> YEHTAVMPNKVGIPYK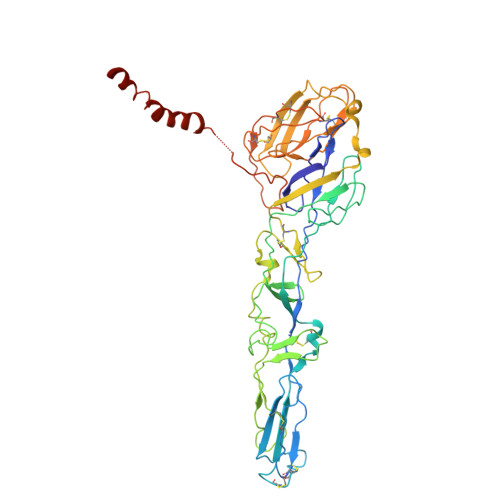ALVERPGYAPVHLQIQLVNTRIIPSTNLEYITCKYKTKVPSPVVKCCGATQCTSKPHPDYQCQVFTGVYPFMWGGAYCFCDTENTQMSEAYVERSEECSIDHAKAYKVHTGTVQAMVNITYGSVSWRSADVYVNGETPAKIGDAKLIIGPLSSAWSPFDNKVVVYGHEVYNYDFPEYGTGKAGSFGDLQSRTSTSNDLYANTNLKLQRPQAGIVHTPFTQAPSGFERWKRDKGAPLNDVAPFGCSIALEPLRAENCAVGSIPISIDIPDAAFTRISETPTVSDLECKITECTYASDFGGIATVAYKSSKAGNCPIHSPSGVAVIKENDVTLAESGSFTFHFSTANIHPAFKLQVCTSAVTCKGDCKPPKDHIVDYPAQHTESFTSAISATAWSWLKVLVGGTSAFIVLGLIATAVVALVLFFHRH> MLEADDQGCIEEQGVEDSANEDSVDAKPDRSSFVPSLFSKKKKNVTMRSIKTTRDRVPTYQYNMNFEKLGKCIIINNKNFDKVTGMGVRNGTDKDAEALFKCFRSLGFDVIVYNDCSCAKMQDLLKKASEEDHTNAACFACILLSHGEENVIYGKDGVTPIKDLTAHFRGDRCKTLLEKPKLFFIQACRGTELDDGIQADSGPINDTDANPRYKIPVEADFLFAYSTVPGYYSWRSPGRGSWFVQALCSILEEHGKDLEIMQILTRVNDRVARHFESQSDDPH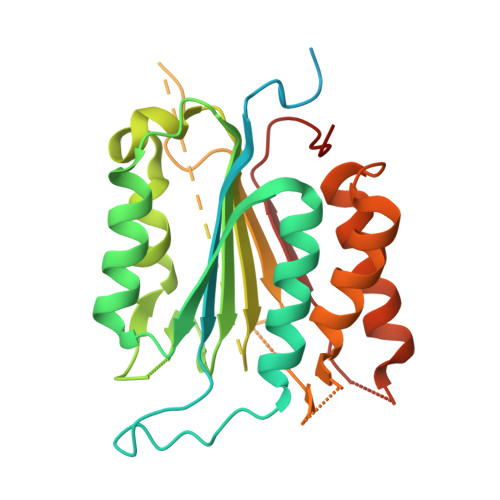FHEKKQIPCVVSMLTKELYFSQ> MADRKLTHFKFFYNTPLTDYQNTIHFSSNNERDNYFLNENHFNAIDYKNIPFNFIRDRNMVNLEQMSWQDAQGINYCTFKSDFENRRYYAFVNQIEYVNDHVTRMYLVIDTVMTYTQGNVLSTVQNAFVERQHLPRDVYNYLLPSLRNNDDVIKASNKYYLNNYLEQFGGNLVLFQSSADLSKKFGTKKEPNLESSKGITYDYITSPVNLYVMNREDFNNFMDKMSKYPWITQNFQKIILIPATFINKDDLEAVKTQEDIKGLMTLKNDKLSNEWELKELRVPFERLQYMLNSNQDELKHLVRNEYL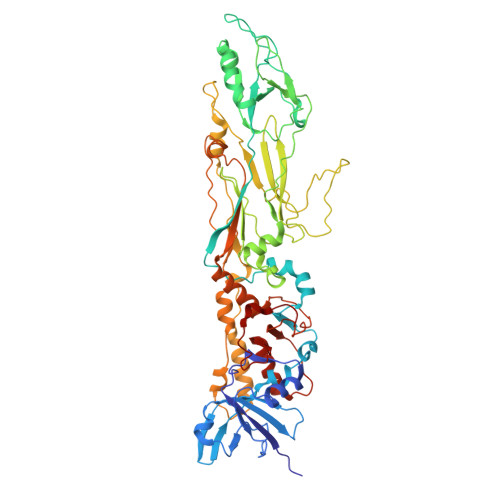TIEIYSWNGDSLLLDAGKITERTGVKLKTKSIIGYHNEVRIYPVDYNSAPNEKPIKASDNSILIDTGSFLNTAITFDSFAEVPILIDNGLLAQSQQANKQKNAQSNLISNRINNVVNGNDLKSRFYDAVSIGSNLSPTALFSKFNDEYNYYKELRAEYKDLALQPPTVTSSQMGNAFQIANSINGLTMKIGVPAPFDMDNIQRYYFMLGFETNDQAGTPFPIDSWTVCNYLRMRGTYTIDGIDPMLLEQLKVLLETGVRFWHNDGTNNPMAQNVFKNKFRK>MPCSEETPAISPSKRARPAEVGGMQLRFARLSEHATAPTRGSARAAGYDLYSAYDYTIPPMEKAVVKTDIQIALPSGCYGRVAPRSGLAAKHFIDVGAGVIDED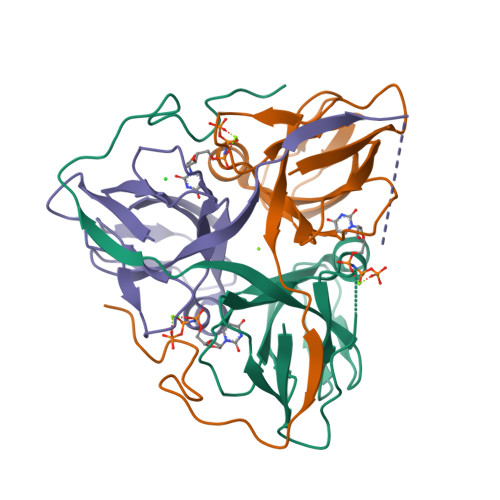YRGNVGVVLFNFGKEKFEVKKGDRIAQLICERIFYPEIEEVQALDDTERGSGGFGSTGKN[3x]>SLINDIILTDDKWLLKNPAWTKKYNEIEQSMPAINDLSQFLKEQNVEFYFALPPSKTNALSFKLPSHIHTYAQENLNYFLKKLPADVKPIKLMEHFKQNYTNEEIQDMYFKTDHHWNMDGAFLGYQYIMNTIGQQSSIYKGKEIAAADYTRTCAQNKHLVGSFNNQLYQLIDANGEKLCYYTPKDGFNFTSVTAKDVQGTVHQNLDEIYGVEAAADTTSYAGYYTDDYPEIVIENNNAQNEVRALVLKDSFANAIVPHLAQSFKHTSILDLRH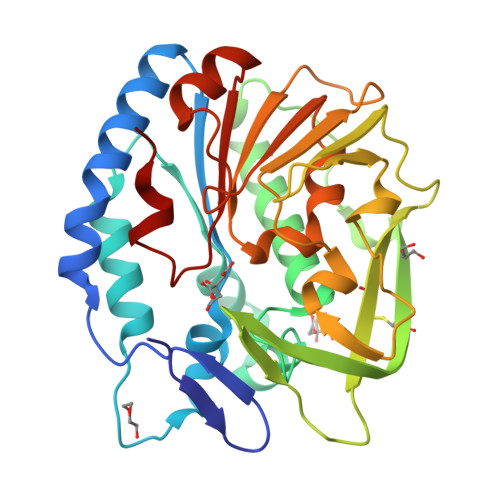YHEKDVYQYIQDNNINMVLFVYSDSNLSGDMFKFKK[2x]> MADADLDKQVNTAGAWPIATGGYYSQHNSPLAQINKSNVKNVKAAWSFSTGVLNGHEGAPLVIGDMMYVHSAFPNNTYALNLNDPGKI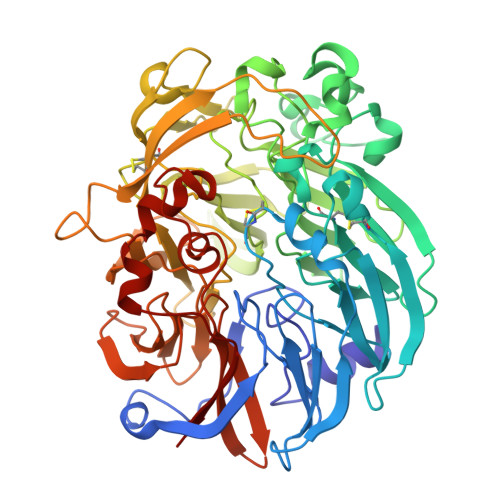VWQHKPKQDASTKAVMCCDVVDRGLAYGAGQIVKKQANGHLLALDAKTGKINWEVEVCDPKVGSTLTQAPFVAKDTVLMGCSGAELGVRGAVNAFDLKTGELKWRAFATGSDDSVRLAKDFNSANPHYGQFGLGTKTWEGDAWKIGGGTNWGWYAYDPKLNLFYYGSGNPAPWNETMRPGDNKWTMTIWGRDLDTGMAKWGYQKTPHDEWDFAGVNQMVLTDQPVNGKMTPLLSHIDRNGILYTLNRENGNLIVAEKVDPAVNVFKKVDLKTGTPVRDPEFATRMDHKGTNICPSAMGFHNQGVDSYDPESRTLYAGLNHICMDWEPFMLPYRAGQFFVGATLAMYPGPNGPTKKEMGQIRAFDLTTGKAKWTKWEKFAAWGGTLYTKGGLVWYATLDGYLKALDNKDGKELWNFKMPSGGIGSPMTYSFKGKQYIGSMYGVGGWPGVGLVFDLTDPSAGLGAVGAFRELQNHTQMGGGLMVFSL4-amino-6-(2,3-difluorophenyl)-7-methyl-7H-pyrrolo[2,3-d]pyrimidine-5-carbonitrile 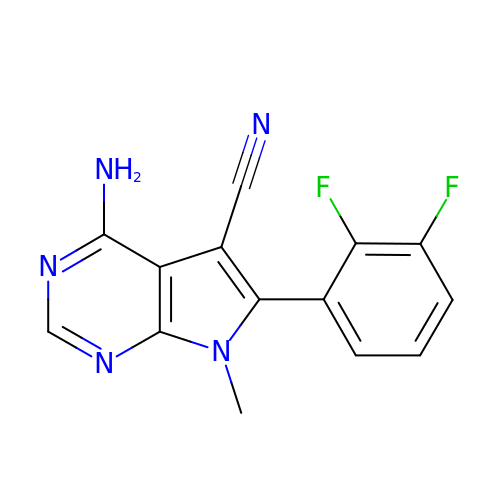| C14 H9 F2 N5 | BGLHMMMVKDNVCA-UHFFFAOYSA-N> MDNYFTAITLLGLRDQNLPPFKDARLQRYKSIKKMIDLIETTTKLAPPMPVELFMLNPTDPEWDDDMTYPTITHATALYKSSALAGNLFLYAYNYNNFTANIRLRTMRYLFPVVSLAIFGNIYWDYRSQL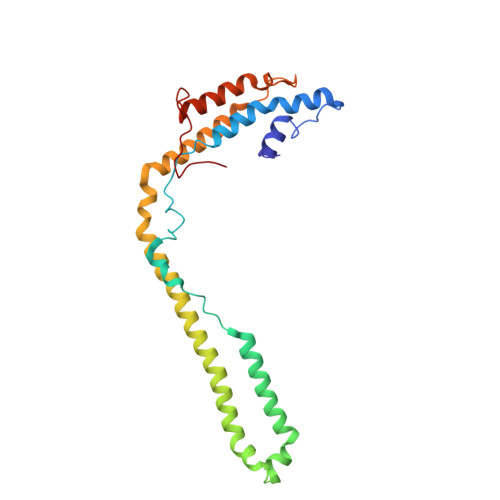VKVNLFDEYIQARAQELVKQNEYLLEHEDVKRYVWWYEDLKETLARVHRQANNHKACDFKDSEIILQDFIRRYTNPKDNLPIKFHPQGQTF> TKPFTLPILTLGELSNSRFPVSIDQMYTSPNEIISVQCQNGRCTLDGELQGTTQLQVSGICAFKGEVTAHLHDNDHLYNVTITNLNGSPFDPSEDIPAPLGVPDFQGRVFGIISQRDKHNSPGHNEPANRGHDAVVPTYTAQYTPKLGQIQIGTWQTDDLTVNQPVKFTPVGLNDTEHFNQWVVPRYAGALNLNTNLAPSVAPVFPGERLLFFRSYIPLKGGYGNPAIDCLLPQEWVQHFYQEAAPSMSEVALVRYINPDTGRALFE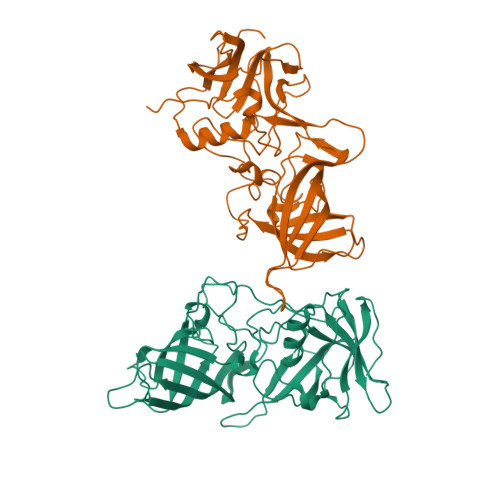AKLHRAGFMTVSSNTSAPVVVPANGYFRFDSWVNQFYSLAPM> MGHHHHHHHHHHSSGHIEGRHMLRERTVRLQYGSRVEAVYVLGTYLWTDVYSAAPAGAQTFSLKHSEHVWVEVVRDGEAEEVATNGKQRWLLSPSTTLRVTMSQASTEASSDKVTVNYYDEEGSIPIDQAGLFLTAIEISLDVDADRDGVVEKNNPKKASWTWGPEGQGAILLVNCDRETPWLPKEDCRDEKVYSKEDLKDMSQMILRTKGPDRLPAGYEIVLYISMSDSDKVGVFYVENPFFGQRYIHILGRRKLYHVVKYTGGSAELLFFVEGLCFPDEGFSGLVSIHVSLLEYMAQDIPLTPIFTDTVIFRIAPWIMTPNILPPVSVFVCCMKDNYLFLKEVKNLVEKTNCELKVCFQYLNRGDRWIQDEIAFGYIEAPHKGFPVVLDSPRDGNLKDFPVKELLGPDFGYVTREPLFESVTSLDSFGNLEVSPPVTVNGKTYPLGRILIGSSFPLSGGRRMTKVVRDFLKAQQVQAPVELYSDWLTVGHVDEFMSFVPIPGTKKFLLLMASTSACYKLFREKQKDGHGEAIMFKGLGGMSSKRITINKILSNESLVQENLYFQRCLDWNRDILKKELGLTEQDIIDLPALFKMDEDHRA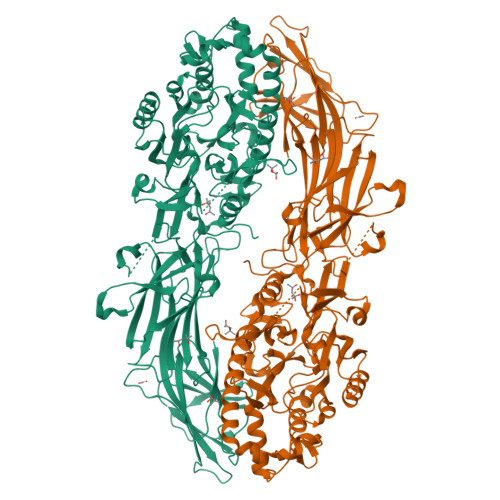RAFFPNMVNMIVLDKDLGIPKPFGPQVEEECCLEMHVRGLLEPLGLECTFIDDISAYHKFLGEVHCGTNVRRKPFTFKWWHMVPSRRS> GPGTRRFERDPTIPPDSIKVYSRTLFLGGITRSVREPVLRSMFERFGSVQSLILNHNYRHGFLKMFRRDAAEKAQVAMENVPFADTTIRTKWGVGFGPRECSDFSTGISVIPIRLLTDADRTWLVTAEYGGTGGLPITPGIALDEPDIEIGLGISSK

The long-wavelength beamline I23 at Diamond Light Source overcomes these limitations and extends the accessible wavelength range to λ = 5.9 Å. In this study, we report the determination of diverse protein structures by experimental phasing techniques carried out at long wavelengths on beamline I23 at Diamond Light Source using S, Ca, K, Cl, V, I, Cd, and P as anomalous scatterers. Native-SAD uses light atoms naturally occurring in proteins or bound to proteins. We demonstrate that long-wavelength native-SAD has become a very compelling technique, where a low multiplicity dataset from a single crystal can be sufficient for successful structure determination, making it a general vehicle of choice for experimental phasing.

To confirm the benefit of collecting at long wavelengths, we collected from Seb1-RRM crystals on beamline I23. A single dataset of 360° from a crystal diffracting to 1.8 Å was sufficient not only to solve the substructure but also to solve the structure without any phase extension, despite the low symmetry space group (C2), low overall completeness (65%) and the 27-fold lower multiplicity of only 6. This case clearly shows that data collection at longer wavelengths requires substantially reduced overall multiplicity. Solving a structure from a single crystal with low multiplicity is advantageous for multiple reasons: the number of crystals might be limited; crystals may not be isomorphous and cannot be merged or they may be especially susceptible to radiation damage.> GSMFTPKPPQDSAVIKAG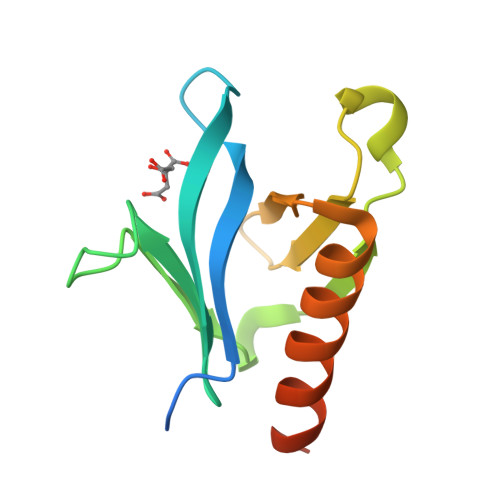YCVKQGAVMKNWKRRYFQLDENTIGYFKSELEKEPLRVIPLKEVHKVQECKQSDIMMRDNLFEIVTTSRTFYVQADSPEEMHSWIKAVSGAIVAQRGPGRSASSEHP AAA+ proteases are a family of proteases that proteolytically cleave substrates from which the substrates are unfolded and delivered to the cleavage sites driven by ATP hydrolysis. Among these AAA+ proteases, FtsH (Filamentation Temperature Sensitive Protein H) is the only known family anchored on membranes where it is able to hydrolyze both soluble and membrane protein substrates. The quality control and regulation of membrane proteins by FtsH play a critical role in cell viability and stress resistance in response to changing environments. FtsHs contain four domains: N-terminal periplasmic and transmembrane domains and C-terminal ATPase and protease domains.

We report here the cryo-EM structure for Thermotoga maritima FtsH (TmFtsH) in a fully ADP-bound symmetric state. We overexpressed the full-length, protease deficient TmFtsH H423Y mutant and purified it in detergents n-Dodecyl-B-D-Maltoside and N,N-Dimethyldodecylamine N-oxide (LDAO) and used negative staining to check particle quality. Therefore, we expressed a membrane scaffold protein MSP1D1 and reconstituted the purified TmFtsH into MSP1D1 nanodiscs in soybean polar lipids. Consequently, our final reconstruction at 3.15 Å resolution used 86,652 particles, consisting only the ATPase and protease domains. The reconstructed map used a six-fold symmetry and displays a higher resolution for the protease domains and lower resolution for the ATPase domains. ADP bound endogenously to TmFtsH and survived the co-purification and reconstitution processes. Our cryo-EM structure may thus represent a fully ADP-bound resting state structure in a six-fold symmetry under physiological conditions. As we used a zinc-binding-deficient mutant H423Y for cryo-EM analysis, we did not model zinc ions in the protease domains. Consequently, the bottom view indicated a shrink of the ATPase pore from the apo to ADP state by a movement of 4.5 Å as measured by the distance between the Cα atoms of residue V235 which is located on the tip of a pore loop. In addition, there are structural changes for the arginine finger in the next clockwise subunit where residue R318′ Cα atom (“R318′” denotes next clockwise subunit) moved 3.6 Å closer to the ADP phosphate groups in the ADP-state structure.

>SNAMNRSNIWNLLFTILIIVTLFWLARFFYVENSPVSKLSYTSFVQMVEDERSVVSEVVIRDDGVLRVYTKDGRVYEVDAPWAVNDSQLIEKLVSKGIKVSGERSGSSSFWINVLGTLIPTILFIVVWLFIMRSLSGRNNQAFTFTKSRATMYKPSGNKRVTFKDVGGAEEAIEELKEVVEFLKDPSKFNRIGARMPKGILLVGPPGTGKTLLARAVAGEANVPFFHISGSDFVELFVGVGAARVRDLFAQAKAHAPCIVFIDEIDAVGRHRGAGLGGGHDEREQTLNQLLVEMDGFDSKEGIIVMAATNRPDILDPALLRPGRFDKKIVVDPPDMLGRKKILEIHTRNKPLAEDVNLEIIAKRTPGFVGADLENLVNEAALLAAREGRDKITMKDFEEAIDRVIAGPARKSKLISPKEKRIIAYYEAGHAVVSTVVPNGEPVHRISIIPRGYKALGYTLHLPEEDKYLVSRNELLDKLTALLGGRAAEEVVFGDVTSGAANDIERATEIARNMVCQLGMSEELGPLAWGKEEQEVFLGKEITRLRNYSEEVASKIDEEVKKIVTNCYERAKEIIRKYRKQLDNIVEILLEKETIEGDELRRILSEEFEKVVE[6x]> TRPFTVPNIPLKYLSNSRIPNPIEGMSLSPDQTQNVQFQNGRCTIDGQPLGTTPVSVSQLCKFRGRITSGQRVLNLTELDGSPFMAFAAPAPAGFPDLGSCDWHIEMSKIPNS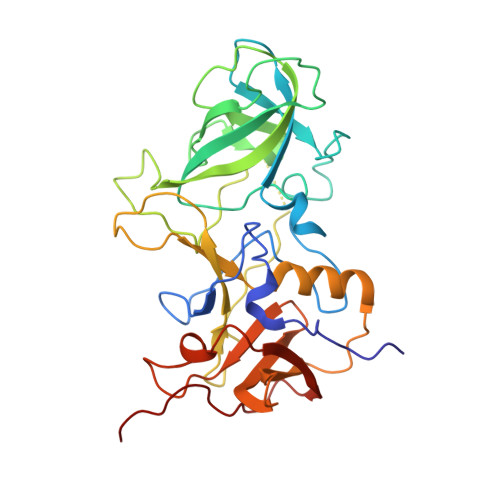STQNNPIVTNSVKPNSQQFVPHLSSITLDENVSSGGDYIGTIQWTSPPSDSGGANTNFWKIPDYGSSLAEASQLAPAVYPPGFNEVIVYFMASIPGPNQSGSPNLVPCLLPQEYITHFISEQAPIQGEAALLHYVDPDTNRNLGEFKLYPGGYLTCVPNSSSTGPQQLPLDGVFVFASWVSRFYQLKPVGTAGPA> GAMVSPSLIAKFEKTSKSNIEGTIKFTPANNGTVSVSVDLKGLPSDIGPFPYHVHEKPVPASKNCSATENHFNPYNGTVRAATPAAHEVGNLAGKHGNIMGESYKTEYDDSYISLNEKS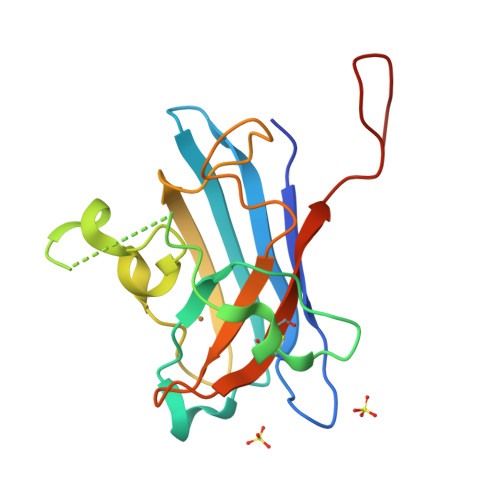RSYIGGLSIVIHANNGTRLNCANITLLDEGHGNANTTMSN> GGGGALPAKENEGCIVSVNSGKRYCLPVGQRSGYSLPDWIVGQEVYVDSGAKAK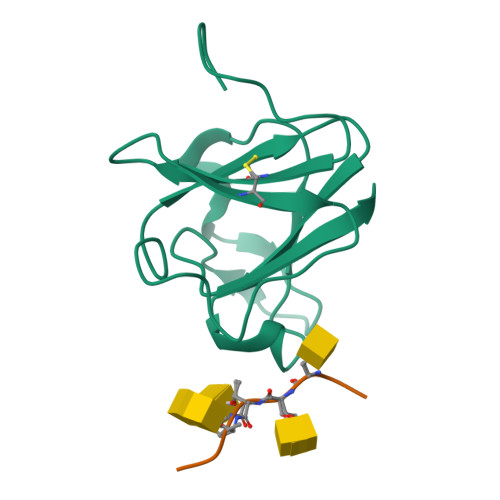VLLSDWDNLSYNRIGEFVGNVNPADMKKVKAWNGQYLDFSKPRSMRVVYK;> AASTTTPAPA> CSLAPDYQRPAMPVPQQFSLSQNGLVNAADNYQNAGWRTFFVDNQVKTLISEALVNNRDLRMATLKVQEARAQYRLTDADRYPQLNGEGSGSWSGNLKGNTATTREFSTGLNASFDLDFFGRLKNMSEAERQNYLATEEAQRAVHILLVSNVAQSYFNQQLAYAQLQIAEETLRNYQQSYAFVEKQLLTGSSNVLALEQARGVIESTRSDIAKRQGELAQANNALQLLLGSYGKLPQAQTVNSDSLQSVKLPAGLSSQILLQRPDIMEAEHALMAANANIGAARAAFFPSISLTSGISTASSDLSSLFNASSGMWNFIPKIEIPIFNAGRNQANLDIAEIRQQQSVVNYEQKIQNAFK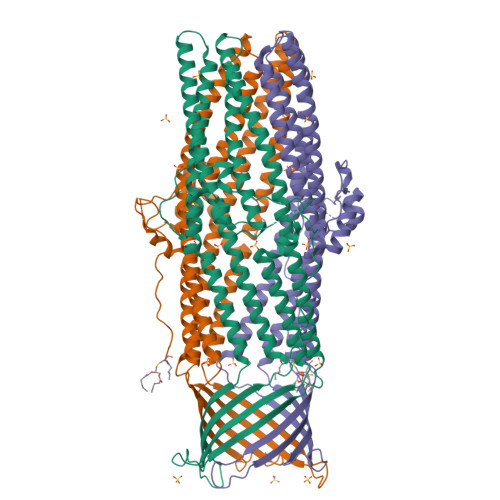EVADALALRQSLNDQISAQQRYLASLQITLQRARALYQHGAVSYLEVLDAERSLFATRQTLLDLNYARQVNEISLYTALGGGHHHHHH>[2x]HMVYPTTLHIIGGQGGNAFSFNGQENAATLQKLSVSVGGWQVRGVQVWLTDGRRETFG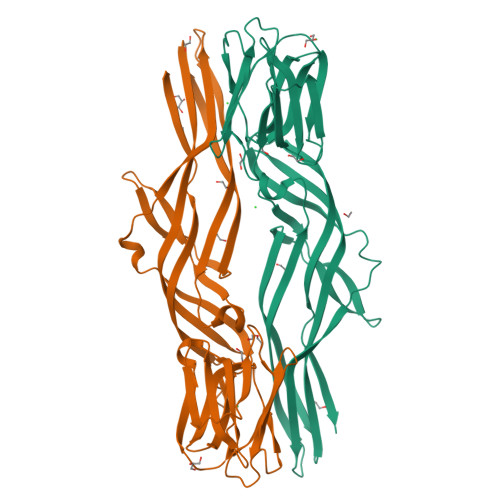AMDSSAKEFEFESGEFIKSLSLWGNGAGTRLGAIKFITSRSREFFAKMTDWGLKTEYKIDVGSGICLGVQGRGGSDIDSMGFIFINAIKSSVIQDMKYPTMHQILPNVQMEEIKEMEYKNDTSIVQSYTFESSKKIIKKSSWSTTNKIESTFSLSVKAGIPEVMEVETGFSFTVGSESTHAVEESEEKTETLTFPVTVPTHKTVTVVANIGRADIDLPYTALLRITCVNGASLDAPLSGIYKGLTYTKMTAVATES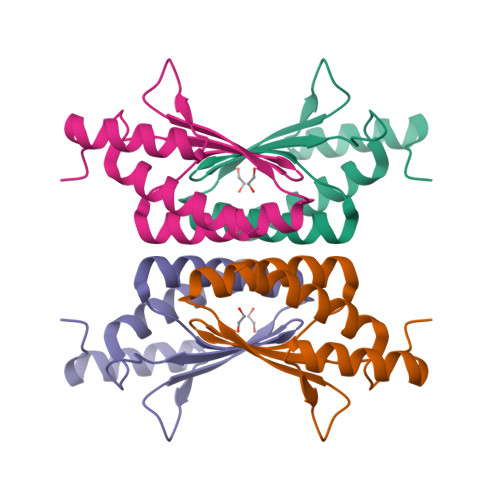> SMSSGTHRLTAEERNQAILDLKAAGWSELSERDAIYKEFSFHNFNQAFGFMSRVALQAEKMNHHPEWFNVYNKVQITLTSHDCGELTKKDVKLAKFIEKAAASV>[2x]MGHHHHHHHHHHSSGHIDDDKHMGGYSMHQLQGNKEYG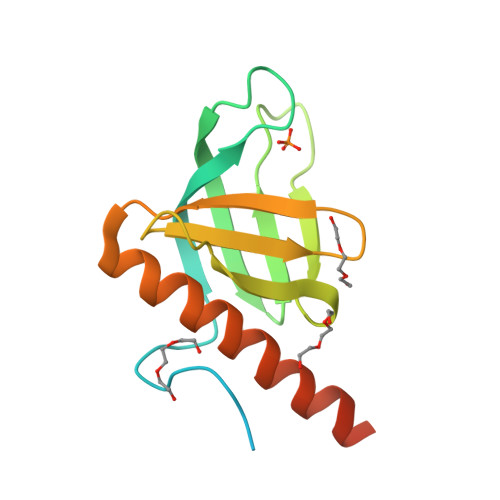SEKKGFLLKKSDGIRKVWQRRKCAVKNGILTISHATSNRQPAKLNLLTCQVKPNAEDKKSFDLISHNRTYHFQAEDEQDYIAWISVLTNSKEEALTMAFRGEQSTGENSLED> GGGGT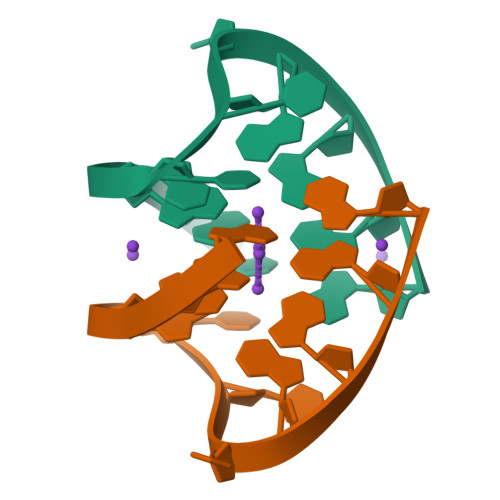TTGGGG> KENALLRYLL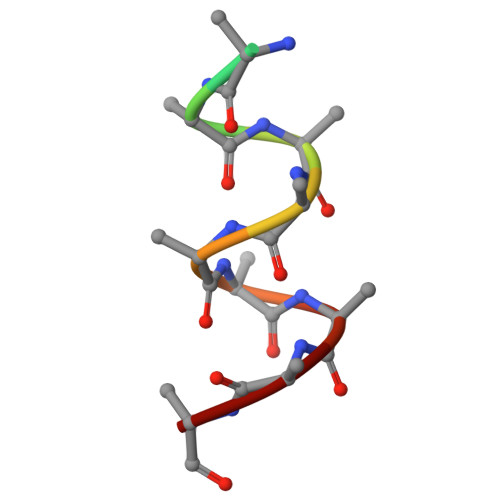DK> XSITKVFARTIFDSRGNPTVEVDLYTSKGLFRAAVPSGASTGVHEALEMRDGDKSKYHGKSVFNAVKNVNDVIVPEIIKSGLKVTQQKECDEFMCKLDGTENKSSLGANAILGVSLAICKAGAAELGIPLYRHIANLANYDEVILPVPAFNVINGGSHAGNKLAMQEFMILPTGATSFTEAMRMGTEVYHHLKAVIKARFGLDATAVGDEGGFAPNILNNKD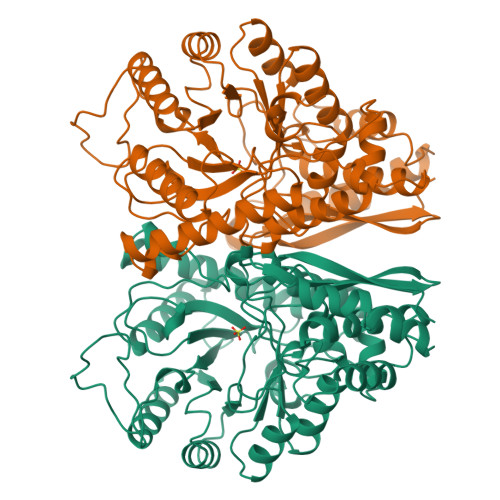ALDLIQEAIKKAGYTGKIEIGMDVAASEFYKQNNIYDLDFKTANNDGSQKISGDQLRDMYMEFCKDFPIVSIEDPFDQDDWETWSKMTSGTTIQIVGDDLTVTNPKRITTAVEKKACKCLLLKVNQIGSVTESIDAHLLAKKNGWGTMVSHRSGETEDCFIADLVVGLCTGQIKTGAPCRSERLAKYNQILRIEEELGSGAKFAGKNFRAPS> MRGSHHHHHHGSKVFVGRCTEDMTAEELQQFFCQYGEVV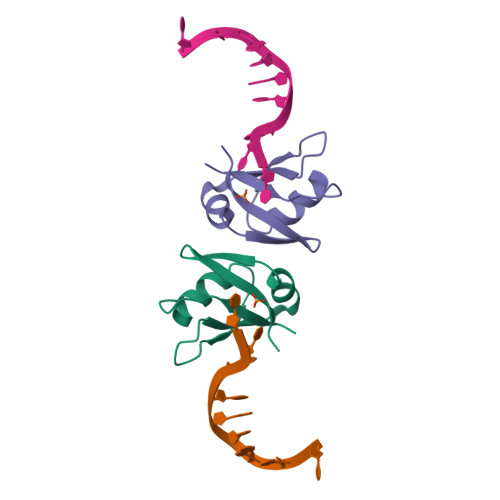DVFIPKPFRAFAFVTFADDKVAQSLCGEDLIIKGISVHISNAEPKHNKLN> ALMTWTAAEFGTNVGFADDQHKTIFDMVNKLHDTAATGNRSEIGKQLDALIDYVVMHFKSEETEMQKKGYADFAAHKAEHDKLVGVCADLQKKFHAGEAEVNQDTTRFVRDWLVNHIPKVDKLY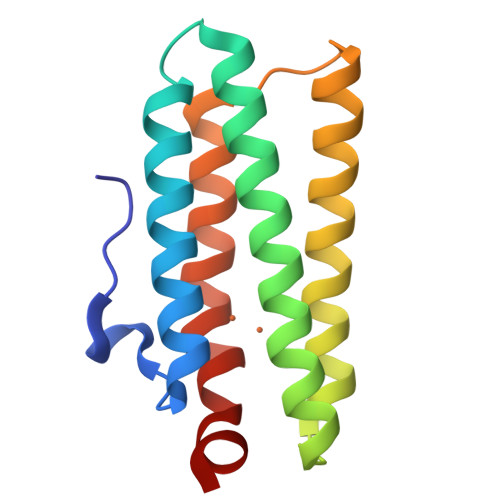GPCLSA>[2x]MGSSLRPLYMDVQATTPLDPRVLDAMLPYLINYYGNPHSRTHAYGWESEAAMERARQQVASLIGADPREIIFTSGATESNNIAIKGVARFYRSRKKHLITTQTEHKCVLDSCRSLEAEGFQVTYLPVQKSGIIDLKELEAAIQPDTSLVSVMTVNNEIGVKQPIAEIGRICSSRKVYFHTDAAQAVGKIPLDVNDMKIDLMSISGHKIYGPKGVGAIYIRRRPRVRVEALQSGGGQERGMRSGTVPTPLVVGLGAACEVAQQEMEYDHKRISKLSERLIQNIMKSLPDVVMNGDPKHHYPGCINLSFAYVEGES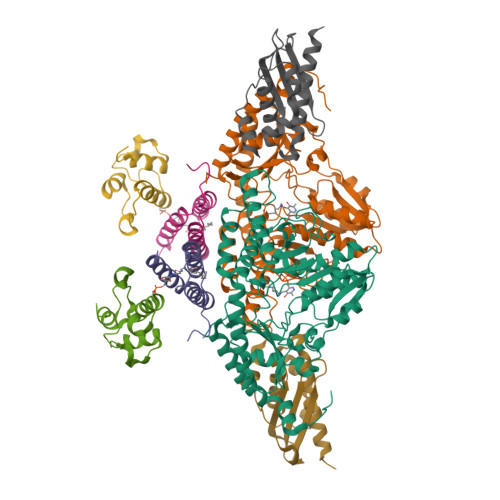LLMALKDVALSSGSACTSASLEPSYVLRAIGTDEDLAHSSIRFGIGRFTTEEEVDYTVEKCIQHVKRLREMSPLWEMVQDGIDLKSIKWTQH;>MAASSRAQVLALYRAMLRESKRFSAYNYRTYAVRRIRDAFRENKNVKDPVEIQTLVNKAKRDLGVIRRQVHIGQLYSTDKLIIENRDMPRT[2x];>[2x]STIEERVKKIIGEQLGVKQEEVTNNASFVEDLGADSLDTVELVMALEEEFDTEIPDEEAEKITTVQAAIDYINGHQA;>[2x]MVLIDMSVDLSTQVVDHYENPRNVGSLDKTSKNVGTGLVGAPACGDVMKLQIQVDEKGKIVDARFKTFGCGSAIASSSLATEWVKGKTVEEALTIKNTDIAKELCLPPVKLHCSILAEDAIKAALADYKLKQEPKKGEAEKKELHHHHHH>[2x]AESHWCYEVQAESSNYPCLVPVKWGGNCQKDRQS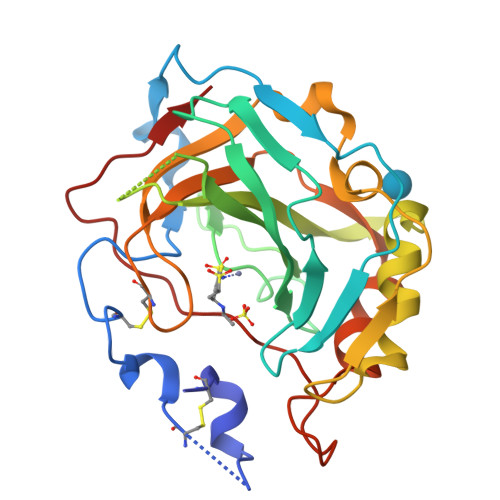PINIVTTKAKVDKKLGRFFFSGYDKKQTWTVQNNGHSVMMLLENKASISGGGLPAPYQAKQLHLHWSDLPYKGSEHSLDGEHFAMEMHIVHEKEKGTSRNVKEAQDPEDEIAVLAFLVEAGTQVNEGFQPLVEALSNIPKPEMSTTMAESSLLDLLPKEEKLRHYFRYLGSLTTPTCDEKVVWTVFREPIQLHREQILAFSQKLYYDKEQTVSMKDNVRPLQQLGQRTVIKS> MNNGEGEVMDLRDIDLNLLVVFNQLLLDRSVSTAGEK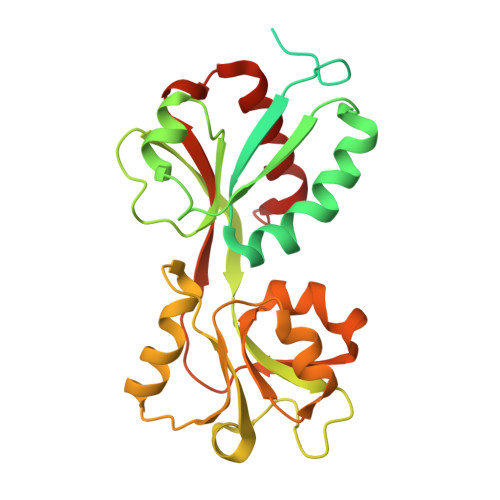LGLTQPAVSNSLKRLRTALNDDLFLRTSKGMEPTPYALHLAEPVIYALNTLQTALTTRDSFDPFASTRTFNLAMTDIGEMYFMPPLMEALAQRAPHIQISTLRPNAGNLKEDMESGAVDLALGLLPELQTGFFQRRLFRHRYVCMFRKDHPSAKSPMSLKQFSELEHVGVVALNTGHGEVDGLLERAGIKRRMRLVVPHFIAIGPILHSTDLIATVPQRFAVRCEVPFGLTTSPHPAKLPDIAINLFWHAKYNRDPGNMWLRQLFVELFSEAHHHHHH> KETA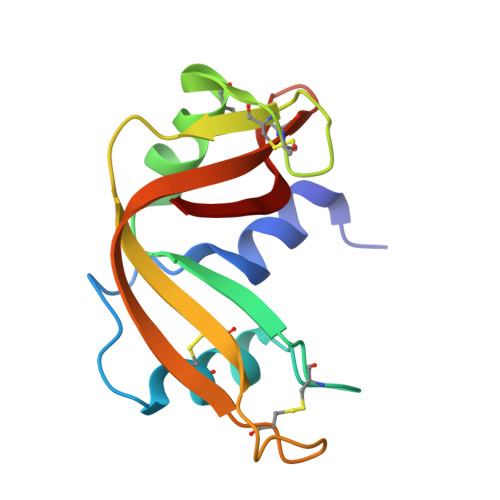AAKFERQHMDSSTSAASSSNYCNQMMKSRNLTKDRCKPVNTLVHESLADVQAVCSQKNVACKNGQTNCYQSYSTMSITDCRETGSSKYPNCAYKTTQANKHIIVACEGNPYVPVHFDASV>[2x]GPERTFIMVKPDGVQRGLVGEVIQRFERRGYKLVAIKMMHASEQLLQTHYEALKSLSFFPKLVAYMSSGPVVPMVFEGRKVVENGRT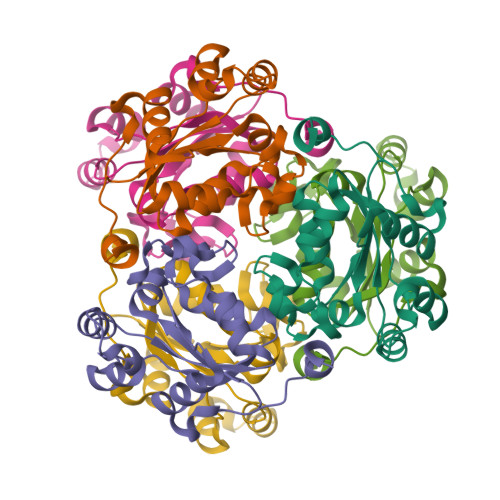MLGATKPEASCPGSIRGDYCQDVGRNVVHGSDSTESANREINLWFSPQELCQYKQAVDPWIHE MM_0014 from the methanogenic archaeon Methanosarcina mazei is known as a versatile cis-prenyltransferase that accepts both isopentenyl pyrophosphate and dimethylallyl pyrophosphate as acceptor substrates. Cis-prenyltransferase (cPT) generally catalyzes the consecutive head-to-tail condensation of isoprene units and produces (Z,E-mixed)-polyprenyl pyrophosphates. MA1831 and MM_0014, which are orthologous cPTs from the methanogenic archaea Methanosarcina acetivorans and Methanosarcina mazei, respectively, unusually accept both IPP and DMAPP as prenyl acceptor substrates. The overall structure of MM_0014 is in a ζ-fold, which is similar to those of so far reported cPTs.

After cleavage of the tag sequence, which should have given the N-terminal sequence starting from GPGYQMDIPKFK where the methionine residue is the putative first residue of native MM_0014, the enzyme was further purified using gel-filtration chromatography and then crystallized in its substrate-free form. The asymmetric unit of the crystal with a C2221 space group contained two protein molecules that comprised a homodimer, which is considered to be the typical biological unit for general cPTs. Subunit A was disordered in the region upstream from Phe6, and subunit B was similarly disordered in this region, but also in the regions between Gly120 and Ile124, between Tyr142 and Lys149, and downstream from Gln213. In each subunit, a β-sheet was composed of parallel β7-β6-β1-β2-β5-β3 strands, and there was an antiparallel β4 strand that existed only in subunit A. The β-sheet was sandwiched by α-helices, and a narrow cavity was formed by α1, α2, α3, and α4 helices and β1, β2, and β5 strands. An inorganic phosphate, which might have been bound throughout the purification process, existed at the opening of the cavity of each subunit. Moreover, a long electron density patch was observed only in the cavity of subunit B. Because the density was thought to be derived from a fatty acid bound to the recombinant enzyme during the expression in the host E. coli cells, palmitic acid was placed provisionally as the ligand because it fit the density well. Although the C-terminus of subunit B was disordered, the C-terminal structure was resolved in subunit A. The C-terminus of subunit A extended toward the cavity of subunit B and covered its cavity opening, where the carboxyl group of the terminal Gly219 residue interacted with a carboxyl oxygen of the purported palmitic acid ligand. In contrast, the cavity of subunit A was in an open conformation because the C-terminus of subunit B was deemed operationally disordered.

>GPGYQMDIPKFKRLPRHIAIIPDGNRRWALARGLEKHEGYSSGIIPGLEVYDICVKIGIGEVTFFGFTQDNTKRPQIQRKAFTDACIKSVQEIAKRDAEILVVGNTNSDIFPEELLEYTKRTKVGKGKIKINFLINYGWYWDLTYAYDNSPDGKKMIENIASAEIPRVDLLIRWGGRCRLSGMLPVQTVYSDIYVVDEMWPDFKPEHLFKALEFYQNQDITLGG[2x]>QPQKRKPKTGILMLNMGGPETLGDVHDFLLRLFLDRDLMTLPIQNKLAPFIAKRLTPKIQEQYRRIGGGSPIKIWTSKQGEGMVKLLDELSPNTAPHKYYIGFRYVHPLTEEAIEEMERDGLERAIAFTQYPQYSCSTTGSSLNAIYRYYNQVGRKPTMKWSTIDRWPTHHLLIQCFADHILKELDHFPLEKRSEVVILFSAHSLPMSVVNRGDPYPQEVSATVQKVMERLEYCNPYRLVWQSKVGPMPWLGPQTDESIKGLCERGRKNILLVPIAFTSDHIETLYELDIEYSQVLAKECGVENIRRAESLNGNPLFSKALAD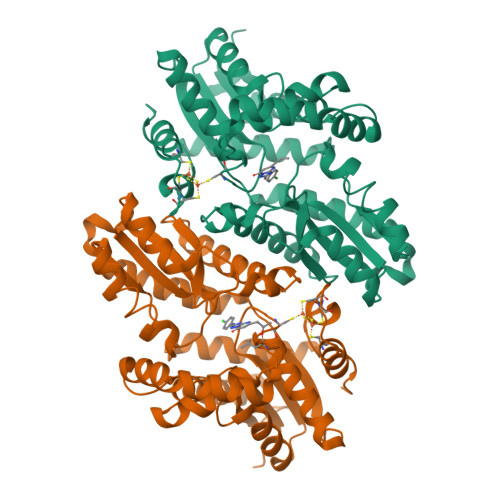LVHSHIQSNELCSKQLTLSCPLCVNPVCRETKSFFTSQQL[2x]>SRKTYTLTDYLKNTYRLKLYSLRWISDHEYLYKQENNILVFNAEYGNSSVFLENSTFDEFGHSINDYSISPDGQFILLEYNYVKQWRHSYTASYDIYDLNKRQLITEERIPNNTQWVTWSPVGHKLAYVWNNDIYVKIEPNLPSYRITWTGKEDIIYNGITDWVYEEEVFSAYSALWWSPNGTFLAYAQFNDTEVPLIEYSFYSDESLQYPKTVRVPYPKAGAVNPTVKFFVVNTDSLSSVTNATSIQITAPASMLIGDHYLCDVTWATQERISLQWLRRIQNYSVMDICDYDESSGRWNCLVARQHIEMSTTGWVGRFRPSEPHFTLDGNSFYKIISNEEGYRHICYFQIDKKDCTFITKGTWEVIGIEALTSDYLYYISNEYKGMPGGRNLYKIQLSDYTKVTCLSCELNPERCQYYSVSFSKEAKYYQLRCSGPGLPLYTLHSSVNDKGLRVLEDNSALDKMLQNVQMPSKKLDFIILNETKFWYQMILPPHFDKSKKYPLLLDVYAGPCSQKADTVFRLNWATYLASTENIIVASFDGRGSGYQGDKIMHAINRRLGTFEVEDQIEAARQFSKMGFVDNKRIAIWGWSYGGYVTSMVLGSGSGVFKCGIAVAPVSRWEYYDSVYTERYMGLPTPEDNLDHYRNSTVMSRAENFKQVEYLLIHGTADDNVHFQQSAQISKALVDVGVDFQAMWYTDEDHGIASSTAHQHIYTHMSHFIKQCFSLP[4x];>MAQTPAFDKPKVELHVHLDGAIKPETILYYGKRRGIALPADTPEELLNIIGMDKPLTLPDFLAKFDYYMPAIAGCRDAIKRIAYEFVEMKAKDGVVYVEVRYSPHLLANSKVEPIPWNQAEGDLTPDEVVSLVNQGLQEGERDFGVKVRSILCCMRHQPSWSSEVVELCKKYREQTVVAIDLAGDE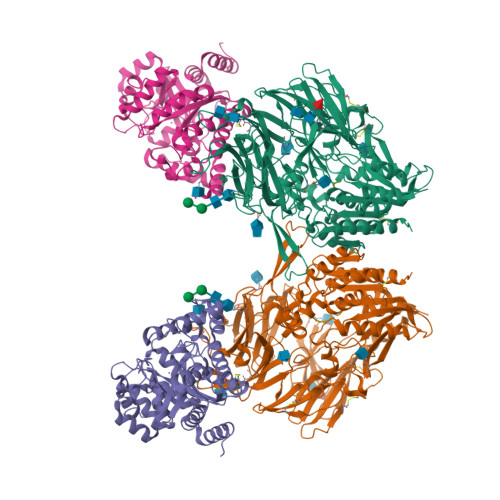TIEGSSLFPGHVQAYAEAVKSGVHRTVHAGEVGSANVVKEAVDTLKTERLGHGYHTLEDTTLYNRLRQENMHFEICPWSSYLTGAWKPDTEHAVIRFKNDQVNYSLNTDDPLIFKSTLDTDYQMTKKDMGFTEEEFKRLNINAAKSSFLPEDEKKELLDLLYKAYRMPSPASAEQCL[4x];>MWPVDPNIE[4x]> HMASLTEIEHLVQSVCKSYRETCQLRLEDLLRQRSNIFSREEVTGYQRKSMWEMWERCAHHLTEAIQYVVEFAKRLSGFMELCQNDQIVLLKAGAMEVVLVRMCRAYNADNRTVFFEGKYGGMELFRALGCSELIS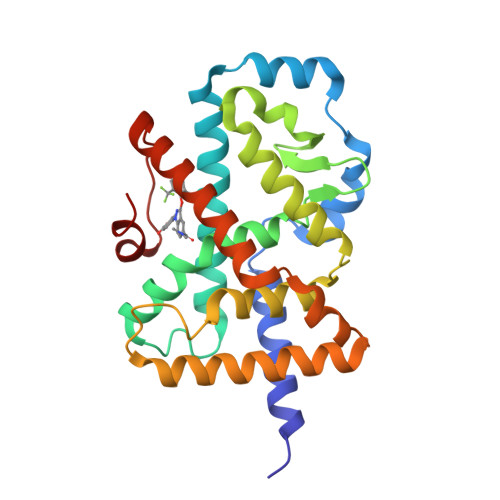SIFDFSHSLSALHFSEDEIALYTALVLINAHRPGLQEKRKVEQLQYNLELAFHHHLCKTHRQSILAKLPPKGKLRSLCSQHVERLQIFQHLHPIVVQAAFPPLYKELF> MAIQRRIRRVKTVQMTTNSPIHRSGSVLEPGNWQEYDPFLLLMEDIFERGTFDVHPHRGIETVTYVISGELEHFDSKAGHSTLGPGDVQWMTAGRGVVHKEDPASGSTVHSLQLWVNLPSAYKMTEPRYQNLRSKDMPVRKEEGATIRVFSGSSKGVKAPTKNIVPVTMVEMIVEPGTTVVQDLPGHYNGFLYILEGSGVFGADNIEGKAGQALFFSRHNRGEETELNVTAREKLRLLLYAGEPVNEPVVAYGPFVMNTPEQIREAIR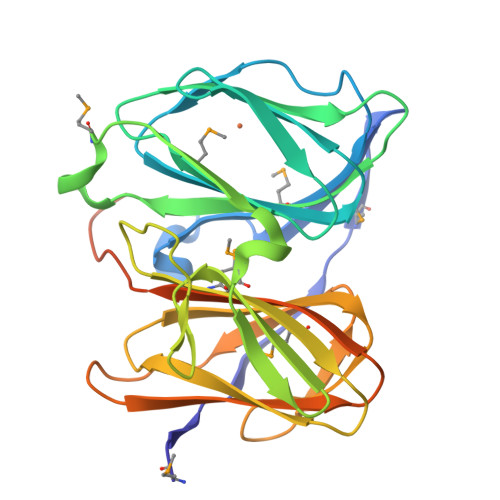DYQEGRFGR>GSHMGQSLRTLQGHQSAVTSLQFNDNIVVSGSDDSTVKVWDIKTGQSLRTLQGHQSAVTSLQFNDNIVVSGSDDSTVKVWDIKTGQSLRTLQGHQSAVTSLQFNDNIVVSGSDDSTVKVWDI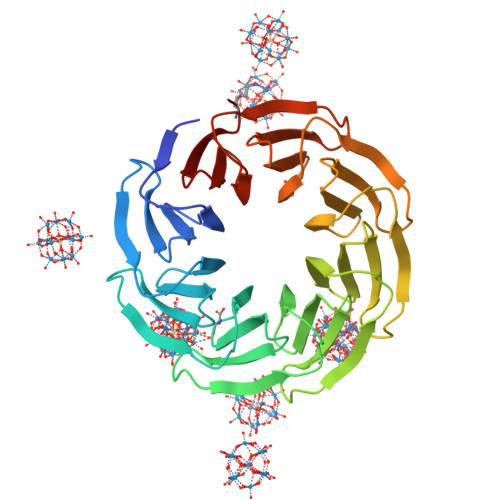KTGQSLRTLQGHQSAVTSLQFNDNIVVSGSDDSTVKVWDIKTGQSLRTLQGHQSAVTSLQFNDNIVVSGSDDSTVKVWDIKTGQSLRTLQGHQSAVTSLQFNDNIVVSGSDDSTVKVWDIKTGQSLRTLQGHQSAVTSLQFNDNIVVSGSDDSTVKVWDIKTGQSLRTLQGHQSAVTSLQFNDNIVVSGSDDSTVKVWDIKT[3x]>MGSSHHHHHHSSGLVPRGSHMASAASYPPIKNTKVGLALSSHPLASEIGQKVLEEGGNAIDAAVAIGFALAVVHPAAGNIGGGGFAVIHLANGENVALDFREKAPLKATKNMFLDKQGNVVPKLSEDGYLAAGVPGTVAGMEAMLKKYGTKKLSQLIDPAIKLAENGYAISQRQAETLKEARERFLKYSSSKKYFFKKGHLDYQEGDLFVQKDLAKTLNQIKTLGAKGFYQGQVAELIEKDMKKNGGIITKEDLASYNVKWRKPVVGSYRGYKIISMSPPSSGGTHLIQILNVMENADLSALGYGASKNIHIAAEAMRQAYADRSVYMGDADFVSVPVDKLINKAYAKKIFDTIQPDTVTPSSQIKPGMGQLHEGSN[2x];>[2x]TTHYSVADRWGNAVSVTYTINASYGSAASIDGAGFLLNNEMDDFSIKPGNPNL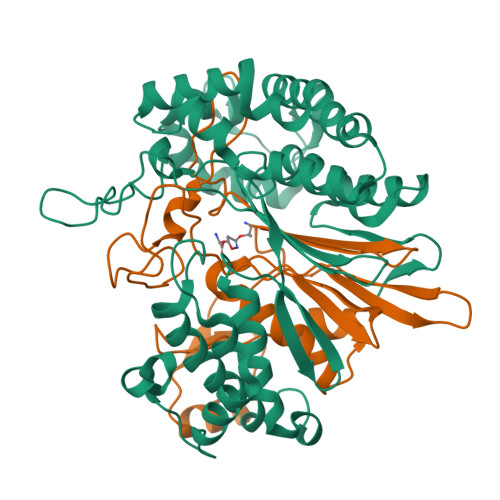YGLVGGDANAIEANKRPLSSMSPTIVLKNNKVFLVVGSPGGSRIITTVLQVISNVIDYNMNISEAVSAPRFHMQWLPDELRIEKFGMPADVKDNLTKMGYQIVTKPVMGDVNAIQVLPKTKGSVFYGSTDPRKEF> PVNPCCYYPCQHQGICVRFGLDRYQCDCTRTGYSGPNCTIPEIWTWLRTTLRPSPSFIHFLLTHGRWLWDFVNATFIRDTLMRLVLTVQSNLIPSPPTYNIAHDYISWESFSNVSYYTRILPSVPRDCPTPMGTKGKKQLPDAEFLSRRFLLRRKFIPDPQGTNLMFAFFAQHFTHQFFKTSGKMGPGFTKALGHGVDLGHIYGDNLERQYQLRLFKDGKLKYQMLNGEVYPPSVEEAPVLMHYPRGIPPQSQMAVGQEVFGLLPGLMLYATIWLREHNRVCDLLKAEHPTWGDEQLFQTARLILIGETIKIVIEEYVQQLSGYFLQLKFDPELLFGAQFQYRNRIAMEFNQLYHWHPLMPDSFRVGPQDYSYEQFLFNTSMLVDYGV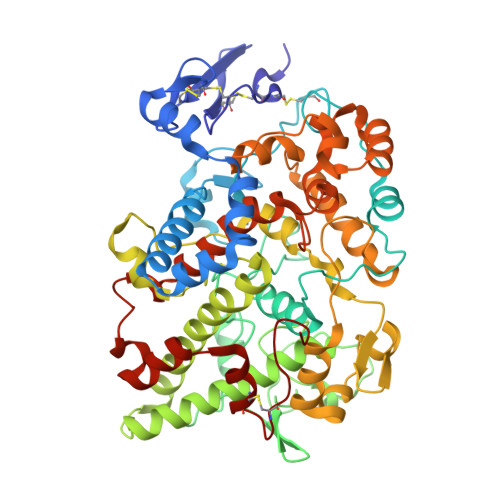EALVDAFSRQPAGRIGGGRNIDHHILHVAVDVIKESRVLRLQPFNEYRKRFGMKPYTSFQELTGEKEMAAELEELYGDIDALEFYPGLLLEKCHPNSIFGESMIEMGAPFSLKGLLGNPICSPEYWKASTFGGEVGFNLVKTATLKKLVCLNTKTCPYVSFHVPD> LLVGGCFVGSRDPNETRYPKAPMPLQNQTSTLKTAEEIRRESVAQN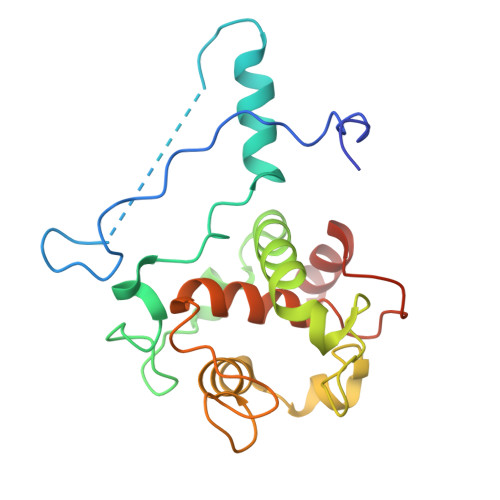TPGAREAAALRDRVTPLNLQQVNEQDVAGNDPLGSPARVVLDEGEMYRDPVEIYREGRALFQNNCVGCHGHNGCGNVPRSTNFTDPGWQENNSDGGIYSSIYNGKGIGNGGGAMPAYYNQLSPQQIRYLVAYLRAFKGRQCNGLPTLSDVERMVAERQ(5R)-4-HYDROXY-3,5-DIMETHYL-5-[(1E,3E)-2-METHYLPENTA-1,3-DIENYL]THIOPHEN-2(5H)-ONE 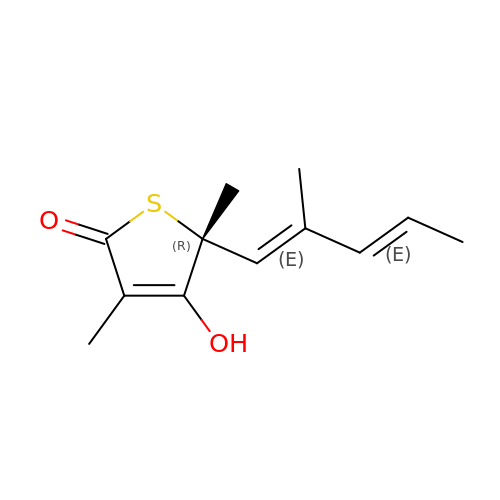| C12 H16 O2 S | FVTQYHVYLPKMOX-SJFBBLFCSA-N>[2x]LVPGEEWEFEVTAFYRGRQVFQQTISCPEGLRLVGSEVGDRTLPGWPVTLPDP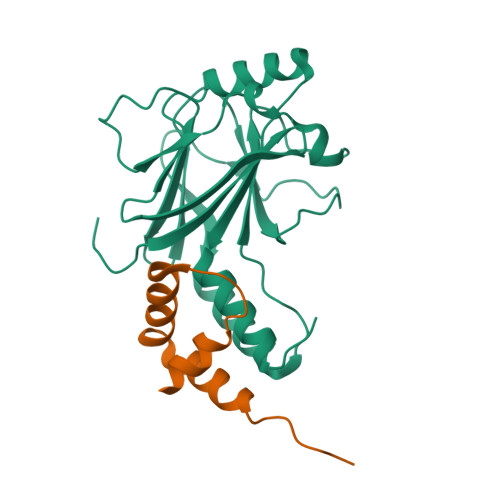GMSLTDRGVMSYVRHVLSCLGGGLALWRAGQWLWAQRLGHCHTYWAVSEELLPNSGHGPDGEVPKDKEGGVFDLGPFIVDLITFTEGSGRSPRYALWFCVGESWPQDQPWTKRLVMVKVVPTCLRALVEMARVGGASS;>[2x]SALQDLLRTLKSPSSPQQQQQVLNILKSNPQLMAAFIKQRTAKYVAN> GCSNISEDVNNPNRSLFLIESEPSTGASVSKNLTEIILIFSNDINKVSQLALTDLITDSDIQGIDYNIEGNKVIINNFSLEPTCNYRLSYEVIDIYDNHLQGYIEFLVNQSNYPQIPDQEVNHTILQAFYWEMNTGEYATEHPEEANLWNLLAERAPELAEAGFTAVWLPPANKGMAGIHDVGYGTYDLWDLGEFDQKGTVRTKYGTKGELENAIDALHNNDIKVYFDAVLNHRMGADYAETVLLDENSRDKPGQYIKAWTGFNFPGRNGEYSNFTWNGQCFDGTDWDDYSKESGKYLFDEKSWDWTYNWDE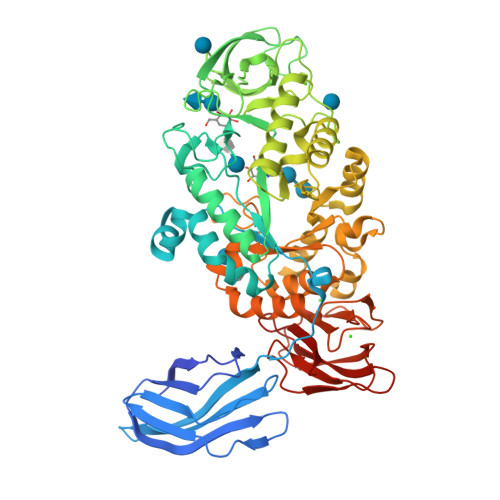DYLMGADVDYENEAVQNDVIDWGQWIINNIDFDGFRLDAVKHIDYRFIDKWMSAVQNSSNRDVFFVGEAWVEDVDDLKGFLDTVGNPDLRVFDFPLRSFFVDMLNGAYMADLRNAGLVNSPGYENRAVTFVDNHDTDRDEGSYTVSIYSRKYQAYAYILTRAEGVPTVYWKDYYIWEMKEGLDKLLTARRYYAYGPGYEVDNNDADIYSYVRSGFPDVAGDGLVLMISDGTSGNVAGKWINSRQPDTEFYDLTGHIKEHVTTDSEGYGNFKVIKSEDKGWSIWVPVE> MAPVRSLNCTLRDSQQKSLVMSGPYELKALHLQGQDMEQQVVFSMSFVQGEESNG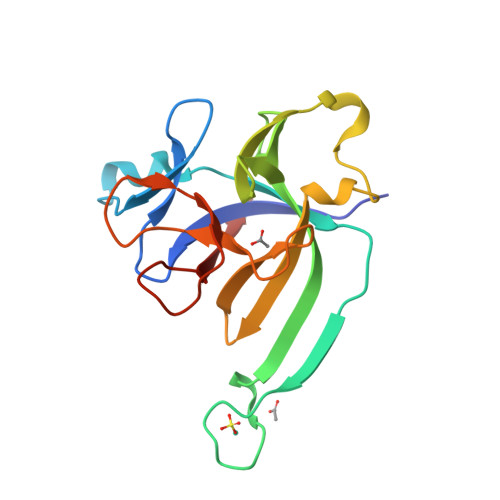YIDTNNDGWIEGDELYDKIPVALGLKEKNLYLSCVLKDDKPTLQLESVDPKNYPKKKMEKRFVFNKIEINNKLEFESAQFPNWYISTSQAENMPVFLGGTKGGQDITDFTMQFVSS>[2x]KIFKPEELRQALMPTLEALYRQDPESLPFRQPVDPQLLGIPDYFDIVKNPMDLST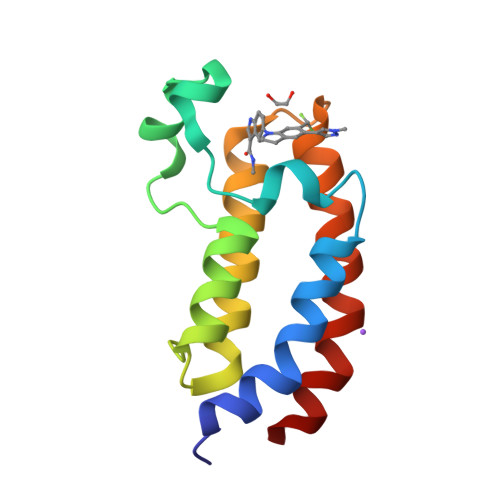IKRKLDTGQYQEPWQYVDDVWLMFNNAWLYNRKTSRVYKFCSKLAEVFEQEIDPVMQSLG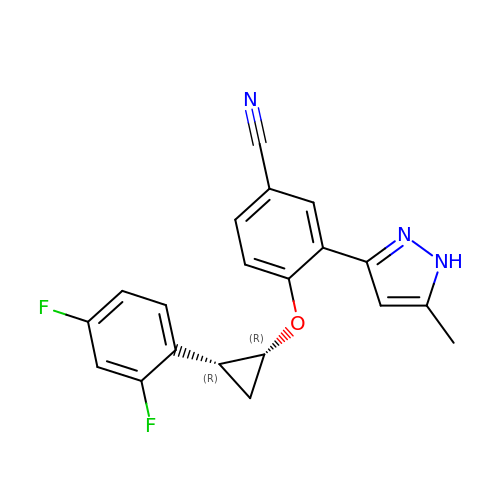4-{[(1R,2R)-2-(2,4-difluorophenyl)cyclopropyl]oxy}-3-(5-methyl-1H-pyrazol-3-yl)benzonitrile | C20 H15 F2 N3 O | QPKQDLGTZJBNKZ-FOIQADDNSA-N>MDKLLLHVGPTTIKEDVLVAGLENNVGFTSKEFVEALAYSLKGLRYVMGASKNYQPLIIPGGGTSAMESVTSLLKPNDKILVV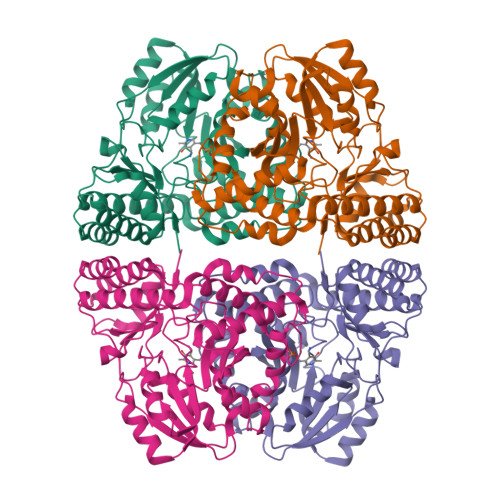SNGVFGDRWEQIFKRYPVNVKVLRPSPGDYVKPGEVEEEVRKSEYKLVALTHVETSTGVREPVKDVINKIRKYVELIVVDGVSSVGAEEVKAEEWNVDVYLTASQKALGSAAGLGLLLLSPKALSILDSQNSIAGYYLDLRNWLPVMRGAEEGKAAYFATPPVHVILQLAEAFRLIEKEGIENRIKRHTMVASAIRAGLEALGLEIVARRPESYSNTVTGVILKVADPQKVLAGTVNEGVEFAPGVHPAFKYFRIGHMGWVTPNDAIIAISVIERTLRKLGEPIRFGEGVKAVEEVLFSAR[2x]>[3x]PYW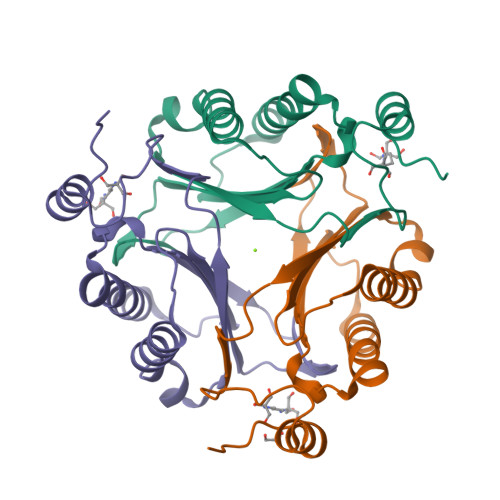EIFTPENAFTPDDKEQLSEAITSIYVDYVNLPRFYVVVLFKDMPKETMYVGGKANNNFVRIRLDHIARQMETAEVRALMMTVAEEKLAPFIKERGYDWEIHIDETPMDLWRTQGLVPPPPESDMEKLWAKENRPIPYD>GSLRKQELVTQNELLKQQVKIFE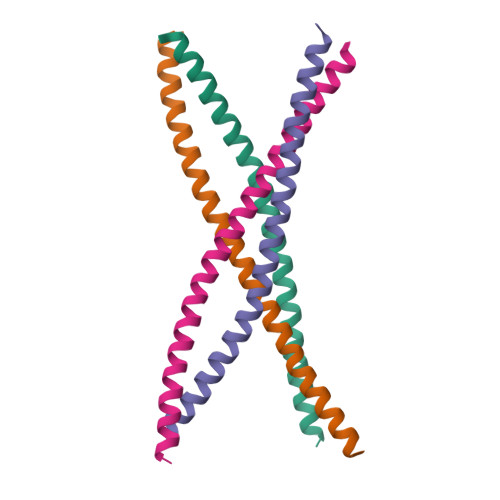EDFQRERSDRERMNEEKEELKKQVEKLQAQVTLTNAQLKTLKEEEKAKE[4x]> GSPSDNSGAEEMEVSLAKPKHRVTMNEFEYLKLLGKGTFGKVILVKEKATGRYYAMKILKKEVIVAKDEVAHTLTENRVLQNSRHPFLTALKYSFQTHDRLCFVMEYANGGELFFHLSRERVFSEDRARFYGAEIVSALDYLHSEKNVVYRDLKLENLMLDKDGHIKITDFGLCKEGIKDGATMKTFCGTPEYLAPEVLEDNDYGRAVDWWGLGVVMYEMMCGRLPFYNQDHEKLFELILMEEIRFPRTLGPEAKSLLSGLLKKDPKQRLGGGSEDAKEIMQHRFFAGIVWQHVYEKKLSPPFKPQVTSETDTRYFDEEFTAQMITITPPDQDDSMECVDSE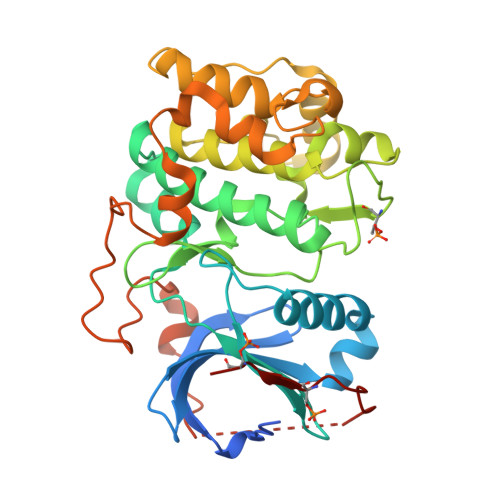RRPHFPQFSYSASGTA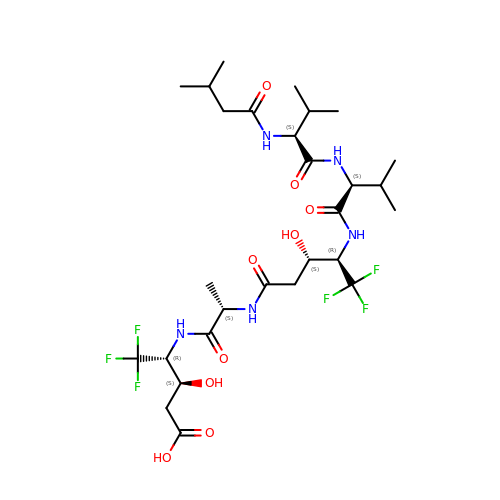5,5,5-TRIFLUORO-3-HYDROXY-4-[2-(5,5,5-TRIFLUORO-3-HYDROXY-4-{3-METHYL-2-[3-METHYL-2-(3-METHYL-BUTYRYLAMINO)-BUTYRYLAMINO]-BUTYRYLAMINO}-PENTANOYLAMINO)-PROPIONYLAMINO]-PENTANOIC ACID | C28 H45 F6 N5 O9 | UDWBPCUKJLZZFA-AIBCRYBESA-N Toxoplasma and Plasmodium are the parasitic agents of toxoplasmosis and malaria, respectively, and use perforin-like proteins (PLPs) to invade host organisms and complete their life cycles. Escape from the PV, and therefore from the infected cell, for subsequent rounds of infection has been shown to be dependent on the perforin-like protein TgPLP1 (T. gondii PLP). We report structures of the membrane attack complex/perforin (MACPF) and Apicomplexan PLP C-terminal β-pleated sheet (APCβ) domains of TgPLP1. The MACPF domain forms hexameric assemblies, with ring and helix geometries, and the APCβ domain has a novel β-prism fold joined to the MACPF domain by a short linker.

We first obtained oligomeric crystal forms of the TgPLP1 MACPF domain by the use of in situ trypsinization in crystallization drops. On solution of the resulting structures, we found two related assemblies: a ring-shaped hexamer and a helical packing arrangement with six subunits per turn. The ring-shaped assembly was, by contrast, found in a C2221 crystal form that diffracted to only 5.0 Å and that we phased by molecular replacement using a single subunit from the P65 crystal form. By contrast, however, the ring-form oligomer crystal structure is imperfect with three main-chain hydrogen bonds being found between only two of the subunit interfaces (“A-B” and “D-E”). Together with the low resolution of the structure, which was only subject to rigid-body refinement, this suggests that the ring-form crystal structure may not represent a functional biological assembly although it may represent an assembly intermediate. In the crystal structures, all subunit interfaces in the helical assembly are identical, but the ring oligomer has three different interfaces, with three, one, and no main-chain hydrogen bonds, respectively, in contrast to the six in each of the helical subunit interfaces. The hydrogen bonds observed in the helical assembly are in a different register to those found in the ring assembly. The ring assembly we observe in the low-resolution crystal form could be an intermediate on the way to the formation of such a helix, but its poor geometry and instability make it a poor candidate for a biologically active structure.

>ETGTVPAINYLGAGYDHVRGNPVGDPSSMGDPGIRPPVLRFTYAQNEDGVSNDLTVLQPLGGYVRQYVACRQSETISELSNLSDYQNELSVDASLQGGDPIGLNSFSASTGYRDFAKEVSKKDTRTYMLKNYCMRYEAGVAQSNHFKWNVTLAFAAGVSQLPDVFDAHNPECACSAEQWRQDQNAEACTKTNVPIWISFIEQFGTHFLVRLFAGGKMTYQVTAKRSEVEKMRNMGIDVKTQLKMQLGGVSGGAGQGTSSKKQQSSSEYQMNVQKETLVIGGRPPGQVSDPAALAAWADTVEELPMPVKFEVQPLYHLLPVEKQEAFKQAVTFYSKAVGLTPQDLSALGTKHHHHHH[6x]> AVPFVEDWDLVQTLGEGAYGEVQLA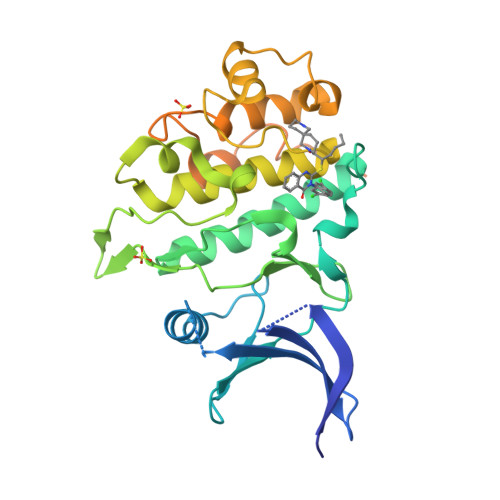VNRVTEEAVAVKIVDMKRAVDCPENIKKEICINKMLNHENVVKFYGHRREGNIQYLFLEYCSGGELFDRIEPDIGMPEPDAQRFFHQLMAGVVYLHGIGITHRDIKPENLLLDERDNLKISDFGLATVFRYNNRERLLNKMCGTLPYVAPELLKRREFHAEPVDVWSCGIVLTAMLAGELPWDQPSDSCQEYSDWKEKKTYLNPWKKIDSAPLALLHKILVENPSARITIPDIKKDRWYNKPLKKGAKRPRVTSGGVSESPSGFSKHIQSNLDFSPVNSASRTPGSGWSKEHHHHHH>[2x]MMVLVTYDVNTETPAGRKRLRHVAKLCVDYGQRVQN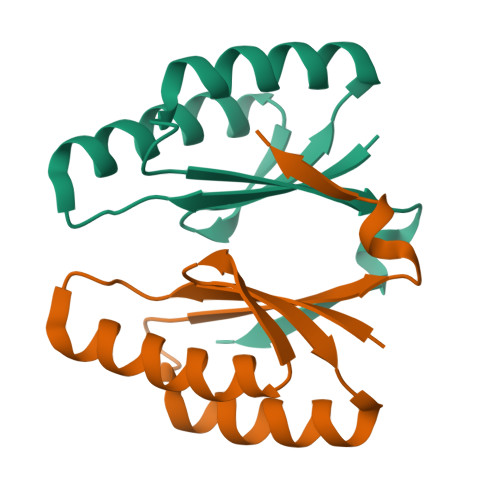SVFECSVTPAEFVDIKHRLTQIIDEKTDSIRFYLLGKNWQRRVETLGRSDSYDPDKGVLLL> MVMTVRVIAPDKTVWDAPAEEVILPSTTGQLGILSNHAPLLTALETGVMRVRQDREWVAIALMGGFAEVENNEVTILVNGAERGDTIDLEKAKAEFAAAQAALAQAEQGESKQAKIQATQAFRRARARLQAAGGVVEI;> MEKTIKDTRKITEAMRLVAAAKVAAAQEQVMASRPFADRLAQVLYSLQTRLRFEDVDLPLLAKRPVKTVALLVVTGDRGLCGGYNTNVIRRAKERLQELEAEGLKYTLVIVGRKAAQYFQRRDYPIDAVYSGLEQIPS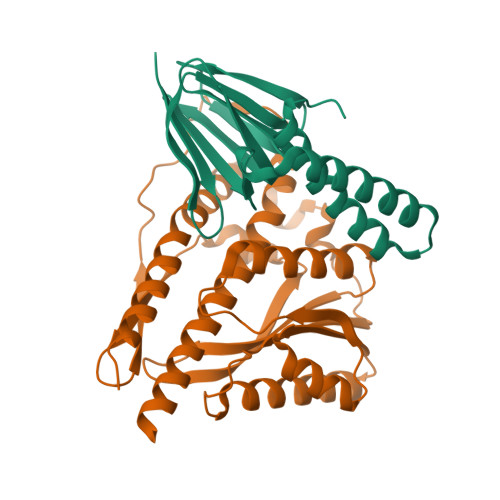ASEAGQIASELLSLFLSETVDRVELIYTKFVSLISSKPVVQTLLPLDPQGLETADDEIFRLTTRGSHLEVNREKVTSTLPALPSDMIFEQDPLQILDALLPLYLNNQLLRALQEAAASELAARMTAMNNASDNAQALILVPR>[2x]GHMNIEALTAELDGIRIEDNEKIVQQKSRDFYWYSPLLKR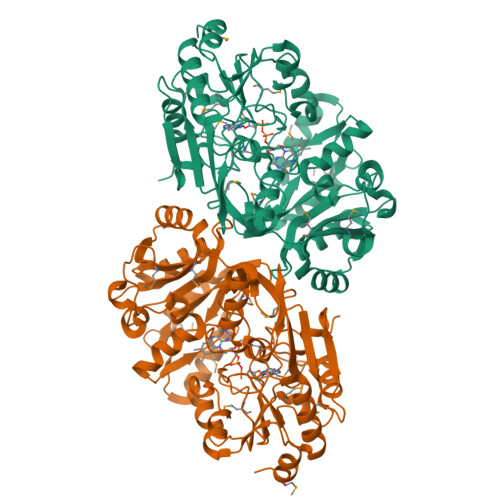QLDHVTGDLVVSPKTEAELIRVLKACYRHEVPVTPRGTGTGNYGQAMPLSGGVVLSLADMNDIREIKPGWVICGPGVICSDLDKAARAHSGQELRMHPSTYHTATVGGFIAGGSGGIGSINWGGLRDFGNIIRLRVVTMEQEPQVLELTGEDLHKVTHAYGTNGIITEIEMPLAPAYDWIDAMVGFDSFDTAAAYANALARQDGILTKLVSVVAAPCPFDYFKRHQKFLKEGQSVVLVMVAAQSHDAFKAFSARSGGEIIFDATTAGDLKGLPPLFELSWNHTTLRALRVDPAWTYLQVLYPFPNQLELTAKMDRMFPGELISHLEFVRFDGDITCFGLPLVKFTTDERLEEIMDLHNANGCPIFNPHRYTLEEGGMKQTDEIQLAFKREADPKGLLNPGKMIAWDDPDYDFNSGKVWLFKGLKQAS> MHHHHHHSSGRENLYFQGMGQEPRTLPPSPNWYCARCSDAVPGGLFGFAARTSVFLVRVGPGAGESPGTP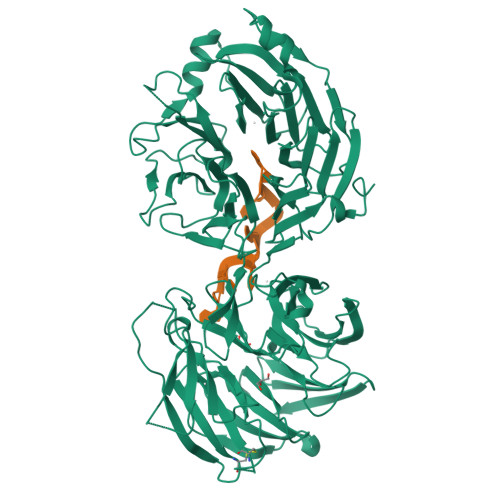PFRVIGELVGHTERVSGFTFSHHPGQYNLCATSSDDGTVKIWDVETKTVVTEHALHQHTISTLHWSPRVKDLIVSGDEKGVVFCYWFNRNDSQHLFIEPRTIFCLTCSPHHEDLVAIGYKDGIVVIIDISKKGEVIHRLRGHDDEIHSIAWCPLPGEDCLSINQEETSEEAEITNGNAVAQAPVTKGCYLATGSKDQTIRIWSCSRGRGVMILKLPFLKRRGGGIDPTVKERLWLTLHWPSNQPTQLVSSCFGGELLQWDLTQSWRRKYTLFSASSEGQNHSRIVFNLCPLQTEDDKQLLLSTSMDRDVKCWDIATLECSWTLPSLGGFAYSLAFSSVDIGSLAIGVGDGMIRVWNTLSIKNNYDVKNFWQGVKSKVTALCWHPTKEGCLAFGTDDGKVGLYDTYSNKPPQISSTYHKKTVYTLAWGPPVPPMSLGGEGDRPSLALYSCGGEGIVLQHNPWKLSGEAFDINKLIRDTNSIKYKLPVHTEISWKADGKIMALGNEDGSIEIFQIPNLKLICTIQQHHKLVNTISWHHEHGSQPELSYLMASGSNNAVIYVHNLKTVIESSPESPVTITEPYRTLSGHTAKITSVAWSPHHDGRLVSASYDGTAQVWDALREEPLCNFRGHQGRLLCVAWSPLDPDCIYSGADDFCVHKWLTSMQDHSRPPQGKKSIELEKKRLSQPKA Among all bacterial pathogens, Legionella pneumophila maintains the largest known set of translocated substrates, delivering over 300 proteins to the host cell via its Type IVB, Icm/Dot translocation system. In at least nine instances, this regulation is direct—a hallmark of an emerging class of proteins called metaeffectors, or “effectors of effectors”. Through detailed structural and functional analysis, we show that metaeffector activity derives from a diverse range of mechanisms, shapes evolution, and can be used to reveal important aspects of each cognate effector's function. After release into the host cell, translocated bacterial substrates (effectors) regulate one another through several different functional interactions: indirectly, through counteracting modification of a shared host target, or directly through either steric complex formation or direct modification of one effector by another.

We next solved the crystal structure of another novel metaeffector, the previously uncharacterized Lpg1148, to reveal a domain (residues 123–304, Table EV4) typical of eukaryotic ubiquitin proteases (UBP) involved in the deconjugation of ubiquitin or ubiquitin‐like proteins from their targets. The de novo crystal structure of the metaeffector LupA (123–304) was determined to 1.9 Å resolution and reveals that LupA belongs to the ubiquitin or ubiquitin‐like protease (UBP) family of proteins with a canonical cysteine protease triad (inset). In vitro activity assays confirmed that Lpg1148 is a ubiquitin‐specific protease whose activity is abrogated by a mutation within the predicted catalytic triad. LupA activity is specific toward ubiquitin. Mutation of a predicted catalytic residue (H183) almost completely abolishes the in vitro hydrolase activity. As Lpg1148 rescues the yeast growth defect caused by LegC3, we hypothesized that this inhibition may derive from the catalytic functionality revealed by our structure. We therefore hypothesized that Lpg1148 (hereafter referred to as Legionella ubiquitin‐specific protease A—LupA) removes a ubiquitin modification from LegC3 that otherwise supports its activity in a proteasomal‐independent manner. LupA activity removes polyubiquitin linkages from its cognate IDTS, LegC3. While polyubiquitination of LegC3 was present when co‐expressed with a catalytically inactive LupA (or in the absence of LupA), no ubiquitination could be detected in the presence of wild‐type LupA, confirming its deubiquitination of LegC3 in vivo. In accordance with our model for LupA metaeffector activity, we detected ubiquitinated species of LegC3 in the presence of catalytically inactive LupA variants but not in the presence of the wild‐type deubiquitinase. These data reveal another novel mechanism of direct effector inactivation—the specific deubiquitination of a cognate effector—and suggest that LegC3 activity may depend upon modification by an endogenous (human) E3 ligase.

>TERDQMQDHDMTLLMPKSQGRIVVMAVLNRYDSHSANAIIETLASDVFNPEVHYIMIPVGPGHWRGVYLSKPQGGTSDTAYDLELFDPYGPEGAAVLDDYVLDLLNQCGVPKELVNIRHTGPKHPQGDAYSCGDFTCAYSHKKMKEFGAPEGSYNPILIDTLDNLGNEDNVLRMTTREETRALVDKDRGR[2x]> NMFCNKEYCNRLKDENNCISNLQVEDQGNCDTSWIFASKYHLETIRCMKGYEPTKISALYVANCYKGEHKDRCDEGSSPMEFLQIIE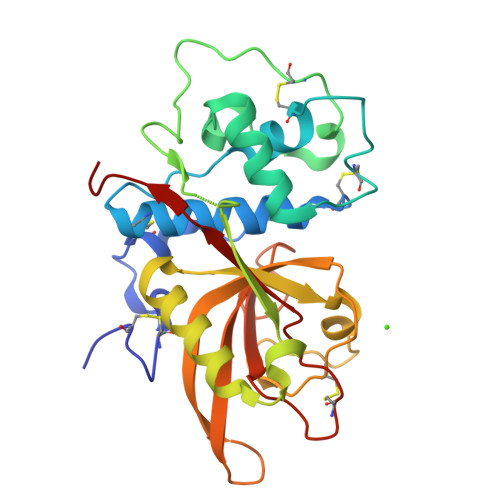DYGFLPAESNYPYNYVKVGEQCPKVEDHWMNLWDNGKILHNKNEPNSLDGKGYTAYESERFHDNMDAFVKIIKTEVMNKGSVIAYIKAENVMGYEFSGKKVQNLCGDDTADHAVNIVGYGNYVNSEGEKKSYWIVRNSWGPYWGDEGYFKVDMYGPTHCHFNFIHSVVIFNVDLPMNN>[3x]MAANKERTFIMV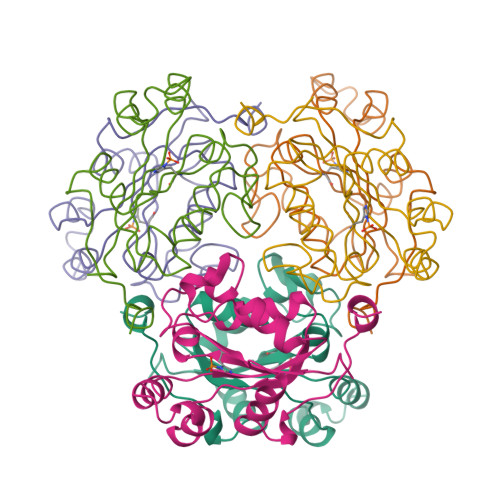KPDGVQRGLVGKIIERFEQKGFKLVALKFTWASKELLEKHYADLSARPFFPGLVNYMNSGPVVPMVWEGLNVVKTGRQMLGATNPADSLPGTIRGDFCIQVGRNIIHGSDAVESAEKEIALWFNEKELVTWTPAAKDWIYE>[2x]GSHMMITMDDIIREGNPTLREVAKEVSLPLSEEDISLGKEMLEFLKNSQDPIKAEELHLR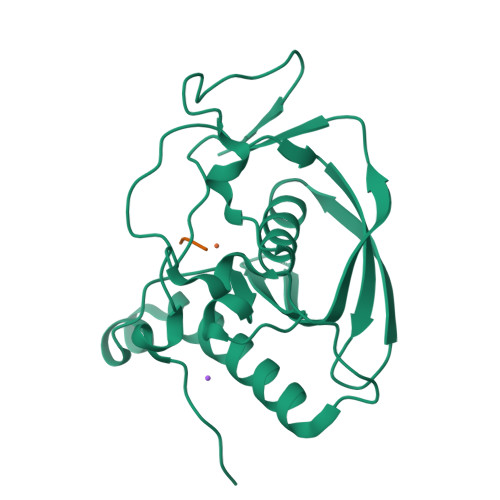GGVGLAAPQLDISKRIIAVHVPSPDPEADGPSLSTVMYNPKILSHSVQDACLGEGEGCLSVDREVPGYVVRHAKITVSYYDMNGEKHKIRLKNYESIVVQHEIDHINGVMFYDHINDQNPFALKEGVLVIE;>MAS[2x]>MRLDVTMRVFNPSYYTAIAEIMKLRSKYITNRSIFVEGSDMVPLLLGLGATRADLDALQRVSNNLYSDPTLPFRRSRNGRFCFDFSTRSVRRLEFQPFALSVEEDFKRHDSGQIRVFDEVQDELQLNTAFQALLVFKGMICHGVQTTHRPRLDYSSDKWVCTLFNLRTVTTPSILGEPALEGVHTDGVDHTMTTYLGSKNMDLAANSAVTFMHDMNEETGAKYTEIKPQNLRSRVQHRHFLDTLLLVDTENKHSLSPVLPLDETKEA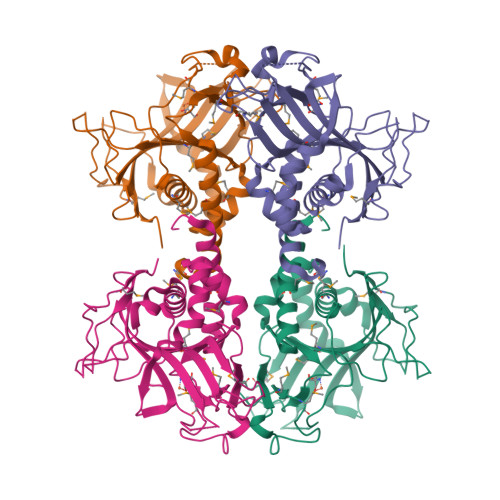TRDMLIFFTRRPVKKGDGGHISENIDSFRPHEELPMEVPLFL[4x]> CIGMIALDAQGNLSGACTTSGMAYKMHGRVGDSPIIGAGLFVDNEIGAATATGHGEEVIRTVGTHLVVELMNQGRTPQQAC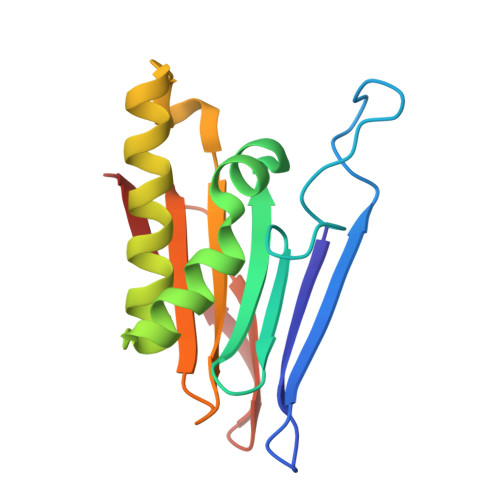KEAVERIVKIVNRRGKNLKDIQVGFIALNKKGEYGAYCIQDGFNFAVHDQKGNRLETPGFALK> KRAMRRYLERGESIEPLDPSEKANKVLARIFKETELRKLKVLGSGVFGTVHKGVWIPEGESIKIPVCIKVIEDKSGRQSFQAVTDHMLAIGSLDHAHIVRLLGLCPGSSLQLVTQYLPLGSLLDHVRQHRGALGPQLLLNWGVQIAKGMYYLEEHGMVHRNLAARNVLLKSPSQVQVADFGVADLLPPDDKQLLYSEAKTPIKWMALESIHFGKYTHQSDVWSYGVTVWELMTFGAEPYAGLRLAEVPDLLEKGERLAQPQICTIDVYMVMVKCWMIDENIRPTFKELANEFTRMARDPPRYLVIKRESGPGIAPGPEPHGLTNKKLE

The HER3 KD functions as an obligate allosteric activator and is itself catalytically inactive, despite high-affinity binding of ATP. The role and relevance of ATP binding for the HER3 KD remains to be defined, but emerging evidence suggests a function in structural stabilization. HER3 is not only essential for tumorigenesis but also functions in mediating drug resistance that becomes apparent when HER2 inhibitors are used to suppress HER2-HER3 signaling.

First, we determined whether displacement of ATP from HER3 KD by high-affinity-binding small molecule ATP analogs, all previously characterized as type I inhibitors, could have an effect. However, none of the small molecules suppressed constitutive HER3 signaling driven by HER2 overexpression. Lack of the inhibitory effect of drug binding on HER3 signaling might be a consequence of the ability of these ATP-mimetic drugs to preserve the same conformation of the HER3 pseudokinase domain as ATP binding. To obtain deeper insights into the effects of drug binding to the HER3 KD, we determined the crystal structure of the HER3 KD/bosutinib complex to a resolution of 2.5 Å. In this structure, HER3 KD adopts the so-called Src/CDK-like inactive conformation, which is the same conformation that HER3 adopts when bound to the ATP analog AMP-PNP (root-mean-square deviation [RMSD] = 0.39 Å). The identical conformational states in the AMP-PNP and bosutinib-bound structures are achieved despite significantly different binding modes employed by bosutinib and the nucleotide. The AP-2 pocket is largely conserved between EGFR and HER3, and it encompasses four hydrophobic residues in HER3: F704, L709, W728, and V786. The pocket adopts a partially open conformation in both the ATP- and bosutinib-bound HER3 structures, stabilized by an edge-to-face π-stacking interaction between F704 and W728. Most importantly, it is connected to K742 in the nucleotide-binding pocket via a network of hydrogen bonds within the β3/β4 strand that extends to V786 in the AP-2 pocket. The side chain of the preceding residue, I741, makes direct hydrophobic interactions with the side chains of L709 and V786.> DPMASVTLSEAEKVYIVHGVQEDLRVDGRGCEDYRCVEVETDVVSNTSGSARVK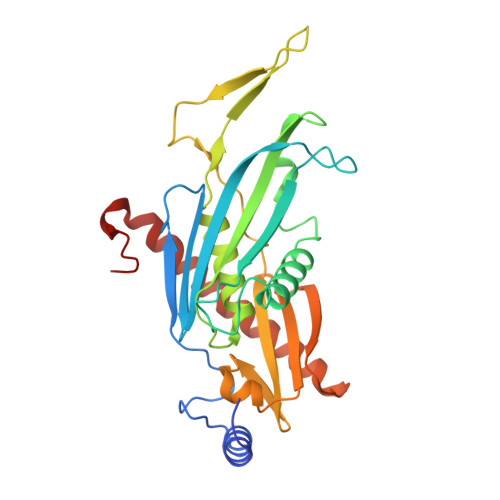LGHTDILVGVKAEMGTPKLEKPNEGYLEFFVDCSASATPEFEGRGGDDLGTEIANTLYRIFNNKSSVDLKTLCISPREHCWVLYVDVLLLECGGNLFDAISIAVKAALFNTRIPRVRVLEDEEGSKDIELSDDPYDCIRLSVENVPCIVTLCKIGYRHVVDATLQEEACSLASLLVSVTSKGVVTCMRKVGKGSLDPESIFEMMETGKRVGKVLHASLQSVVHKEESLGPKRQKVGFLG>[2x]MKNNN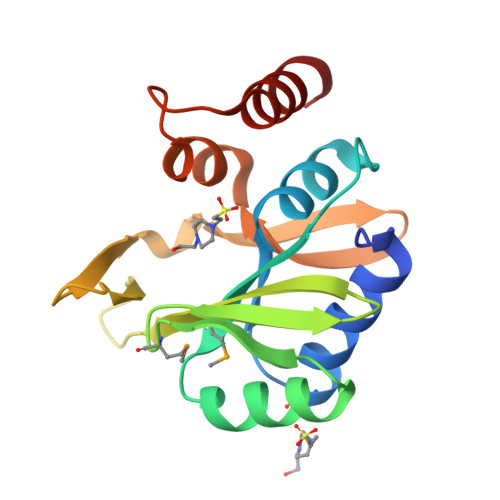VTEKELFYILDLFEHMKVTYWLDGGWGVDVLTGKQQREHRDIDIDFDAQHTQKVIQKLEDIGYKIEVHWMPSRMELKHEEYGYLDIHPINLNDDGSITQANPEGGNYVFQNDWFSETNYKDRKIPCISKEAQLLFHSGYDLTETDHFDIKNLKSIT>MLGIPLLTRKAALTPPAPSANPAKIFIRRFFSAGVAKNVVSYSNVMAAQRAMEHPVAFRCLDKLGLTVQSVKWDVGKDPQNTQVGDGGMSASQRKALQQILQRPNPTMSGAQLRYSAALSWACFGRMAFKVSVMSDGSVNAIWPLGIPFLKQKFDRYGDVESFQYGDEAGKETIPSFTKVEKNDKGRPIKNYAFMIVKPSINGAMNFDVQNTPLQAIGVPVALYDALMARAIDSADGTPNSKWLVTASRDLDDGQAKEVKEGIEETKPGGDNGGEIIFIAGTDVKVQEMKNDLSDIHSKVPLDDQARTIAGNFGIPIALLGFAGADGSKFANNYDESRKAFFEDTIEPGYLTPLEDGFSMFLCGAGYRVIFDRDSIPALRKSRADIAATYDKVTFITEEEKREVTGWPAKKEGQTQNDDA[12x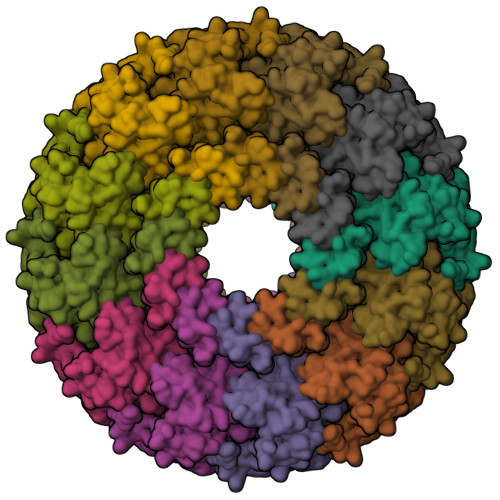]> MRGSHHHHHHENLYFQGSLAVAEPVVNAADAKGTNVNDKVTASDFKLEKTAFDPNQSGNTFMAANFKVTGQVKSGDYFTAKLPDSVTGNGDVDYSNSNNTMPIADIKSTNGDVVAKATYDILTKTYTFVFTDYVNDKENINGQFSLPLFTDRAKAPKSGTYDANINIADEMFDNKITYNYSSPIAGIDKPNGANISSQIIGVDTASGQNTYKQTVFVNPKQRVLGNTWVYIKGYQDKIEESSGKVSATDTKLRIFEVNDTSKLSDSYYADPNDSNLKEVTGEFKDKISYKYDNVASINFGDINKTYVVLVEGHYDNTGKNLKTQVIQENIDPATGKDYSIFGWNNENVVRYGGGSADGDSAVN;> ASGSSGTGSTGNQ

ClfB, an MSCRAMM (Microbial Surface Components Recognizing Adhesive Matrix Molecules) family surface protein, described as a fibrinogen-binding clumping factor, is a key determinant of S. aureus nasal colonization, but the molecular basis for ClfB-ligand recognition remains unknown. ClfB plays a key role in establishing human nasal colonization by binding to the human type I cytokeratin 10 (CK10) expressed on squamous epithelial cells. As a bifunctional MSCRAMM, ClfB also binds to fibrinogen α (Fg α), which is assumed to be significant in platelet activation and aggregation and has been shown to contribute to the pathogenesis of experimental endocarditis in rats. In this study, we solved the crystal structures of apo-ClfB and its complexes with fibrinogen α (Fg α) and cytokeratin 10 (CK10) peptides.

To study the molecular mechanisms underlying ClfB-ligand recognition, we solved the crystal structures of ClfB(208–542) in complex with CK10 (amino acids 499–512, referred as CK10(499–512)) or Fg α (amino acids 316–328, referred as Fg α(316–328)) at 2.3 Å and 1.92 Å, respectively. The structure of the ClfB(208–540)-Fg α(316–328) complex was solved by a Se-Met derived protein and was used as a starting model for determination of the other structures by the molecular replacement method. In both complexes, the peptides adopt an extended conformation and are inserted into the tunnel formed between N2 and N3. In ClfB-Fg α(316–328), the residues ClfBArg529- Ser542 that are disordered in the structure of apo-ClfB become well defined following Fg α(316–328) binding. The distal C-terminus of ClfB(197–542) forms a short β-strand G′, which forms a parallel β-sheet with the β-strand E from the N2 domain. The ligand-induced stabilization of the C-terminal peptide of ClfB allows it to run across Fg α(316–328) on the top. This binding mode is consistent with the DLL model as demonstrated in SdrG-Fg β complex. A sharp twist at Fg αGly318 allows the N-terminal portion of the peptide to exit the tunnel and point upward. Taking the Fg α(316–328)-ClfB complex as an example, within this motif, the G1 is limited by the side chain of ClfBW522 with the limitation of the space and is also required for the Fg α peptide making a turn thus exiting the tunnel. The S2 is the most critical residue because it not only forms two hydrogen bonds with the side chains of ClfBW522 and ClfBQ377 but also binds to the main chain of ClfBS376.>GPHMRYVEIHRNLKGLRKYMAEQAKTNLKLKQRMGDMRREIRKSVGQLTTGGMAANKDKQQKIKSILTEALSNQVESALVDPNNFVVEPRKPVEGATNNDPLLPSIFVYLINIFAKAAISQFINEAGARPETADPVGICVAAILSEPDFLWRGASLIDILIAKFRIVCPVLFGYRGSEKTEQGRQRLGWWKESGQWISEQQHMDRMTGLGAGFAAISLRKFALSKKQNPYPPRFYWMAMAKIVNTPPAEISNTQCVVLKAMVQNYEAKFIEFYGSAAIAALRTALIDFPARAPHKSAAVNSLEVLAQMLKRDT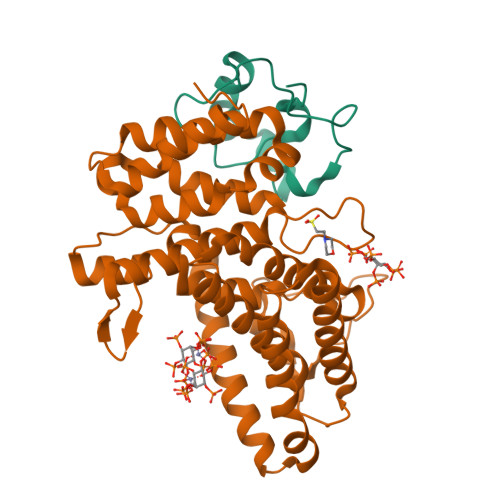GLDLG[2x];>GPHMGSPEFDGTLVRIWMPDGAPAYTADTEAEDPKVYEDEGVKRQWQSFLEKGRFEGGMPEVPPRREWCVWDF[2x]> DAVQKMLGHCTFEPAEPKAAKNTYTAERFIWLTKLNNLRILEQGSERPLTDTER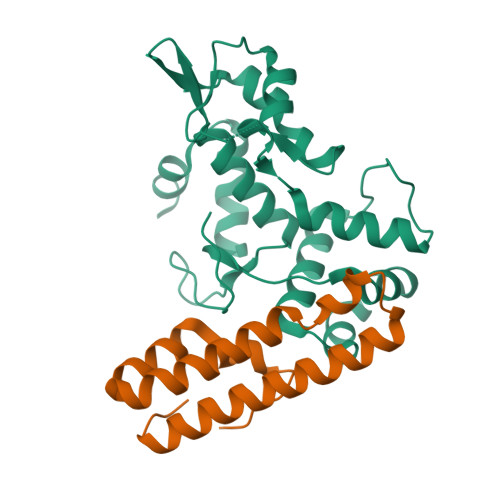ATLMDEPYRKSKLTYAQARKLLGLEDTAFFKGLRYGKDNAEASTLMEMKAYHAISRALEKEGLKDKKSPLNLSPELQDEIGTAFSLFKTDEDITGRLKDRIQPEILEALLKHISFDKFVQISLKALRRIVPLMEQGKRYDEACAEIY;> MKITSSNFATIATSENFAKLSVLPKNHREPIKGLFKSAVEQFSSARDFFKNENYSKELAEKFNKEAVNEAVEKLQKAIDLAEKQGIQF> GPGHKYKKQFRYESQLQMVQVTGSSDNEYFYVDFREYEYDLKWEFPRENLEFGKVLGSGAFGKVMNATAYGISKTGVSIQVAVKMLKEKADSSEREALMSELKMMTQLGSHENIVNLLGACTLSGPIYLIFEYCCYGDLLNYLRSKREKFSEDEIEYENQKRLEEEEDLNVLTFEDLLCFAYQVAKGMEFLEFKSCVHRDLAARNVLVTHGKVVKICDFGLARDIMSDSNYVVRGNARLPVKWMAPESLFEGIYTIKSDVWSYGILLWEIFSLGVNPYPGIPVDANFYKLIQNGFKMDQPFYATEEIYIIMQ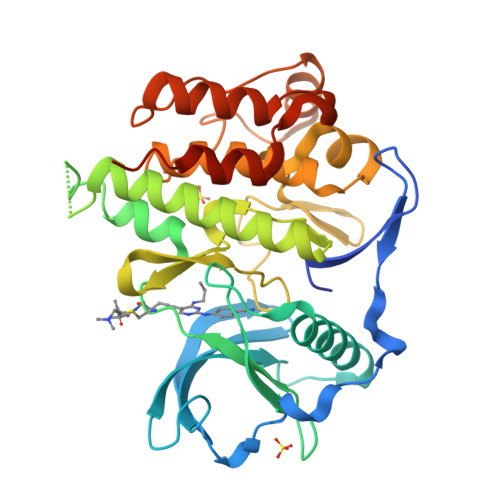SCWAFDSRKRPSFPNLTSFLGCQLADAEEAMYQNV2-{(S)-(2-chlorophenyl)[3-(piperidin-1-yl)propoxy]methyl}-1H-pyrrolo[3,2-b]pyridine-7-carboxylic 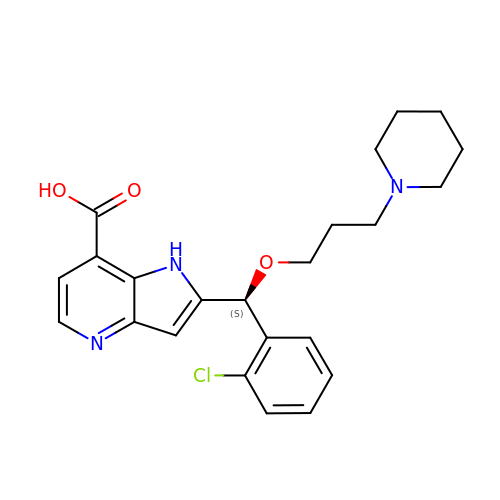acid | C23 H26 Cl N3 O3 | MNARMTUGWVPRGA-QFIPXVFZSA-N>MGSSHHHHHHSSGRENLYFQGMATITLERDGLQLVGTREEPFGEIYDMAIIFHGFTANRNTSLLREIANSLRDENIASVRFDFNGHGDSDGKFENMTVLNEIEDANAILNYVKTDPHVRNIYLVGHAQGGVVASMLAGLYPDLIKKVVLLAPAATLKGDALEGNTQGVTYNPDHIPDRLPFKDLTLGGFYLRIAQQLPIYEVSAQFTKPVCLIHGTDDTVVSPNASKKYDQIYQNSTLHLIEGADHCFSDSYQKNAVNLTTDFLQNNNAF[2x]

We previously showed that LJ0536, a cinnamoyl esterase purified from L. johnsonii N6.2, is active towards a variety of substrates including short acyl chain aliphatic esters and phenolic esters. The structure showed a canonical α/β fold characteristic of esterases, and the enzyme is dimeric. Two classical serine esterase motifs (GlyXSerXGly) can be recognized from the amino acid sequence, and the structure revealed that the catalytic triad of the enzyme is formed by Ser106, His225, and Asp197, while the other motif is non-functional. The structure revealed a prominent inserted α/β subdomain of 54 amino acids, from which multiple contacts to the aromatic acyl groups of the substrates are made.

We determined the structure of the active site mutant (Ser106Ala mutant) and also co-crystallized this mutant with ferulic acid, ethyl ferulate, or chlorogenic acid. As well, no clear electron density was resolved for the quinic acid moiety of chlorogenic acid (labeled as caffeic acid-bound), perhaps due to residual enzymatic activity, or a lack of productive interactions with the enzyme. The caffeic acid moiety of chlorogenic acid adopts a similar position and interaction with the catalytic pocket, as does ferulic acid. However, caffeic acid has two hydroxyl groups in the benzyl ring (positions 3 and 4) which interact with the side chain of Asp138 and Tyr169 through hydrogen bonding. The 4-hydroxyl group (ethyl ferulate, ferulic acid, and caffeic acid) and 3-hydroxyl group (caffeic acid) of the aromatic ring of the substrates are hydrogen bonded to Asp138 and Tyr169, respectively, from the inserted α/β subdomain at the back of the enzyme cavity. The 3-methoxy (3-hydroxyl in the case of caffeic acid) and 4-hydroxyl groups also interact with an ordered water molecule in all of the complexes. This water is also coordinated by the Oγ1 atom of Thr144 from the inserted α/β subdomain. Conversely, functionalities beyond the ester group, including the alkoxyl group of ethyl ferulate/ferulic acid and the quinic acid moiety of chlorogenic acid, appear not to play roles in substrate binding. This notion is suggested due to the fact that we did not observe electron density for the quinic acid moiety of chlorogenic acid, although the binding cleft is large enough to accommodate this group.>[2x]GHM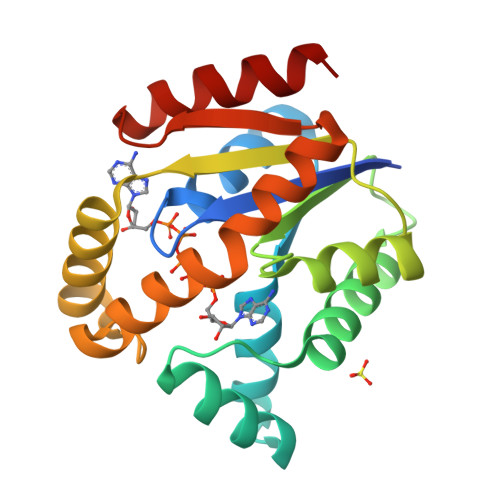ADKIKDAKIIFVVGGPGSGKGTQCEKIVAKYGYTHLSSGDLLRAEVSSGSERGKQLQAIMQKGELVPLDTVLDMIKDAMIAKADVSKGYLIDGYPREVKQGEEFEKKIGKPCLLLYVDAKGETMVKRLMKRGETSGRADDNEETIKKRLDLYYKATEPVIAFYEGRGIVRKVDSELPVDEVFKQVSTAIDAL> MALEVGDMEDGQLSDSDSDMTVAPSDRPLQLPKVLGGDSAMRAFQNTATACAPVSHYRAVESVDSSEESFSDSDDDSCLWKRKRQKCFNPPPKPEPFQFGQSSQKPPVAGGKKINNIWGAVLQEQNQDAVATELGILGMEGTIDRSRQSETYNYLLAKKLRKESQEHTKDLDKELDEYMHGGKKMGSKEEENGQGHLKRKRPVKDRLGNRPEMNYKGRYEITAEDSQEKVADEISFRLQEPKKDLIARVVRIIGNKKAIELLMETAEVEQNGGLFIMNGSRRRTPGGVFLNLLKNTPSISEEQIKDIFYIENQKEYENKKAARKRRTQVLGKKMKQAIKSLNFQEDDDTSRETFASDTNEALASLDESQEGHAEAKLEAE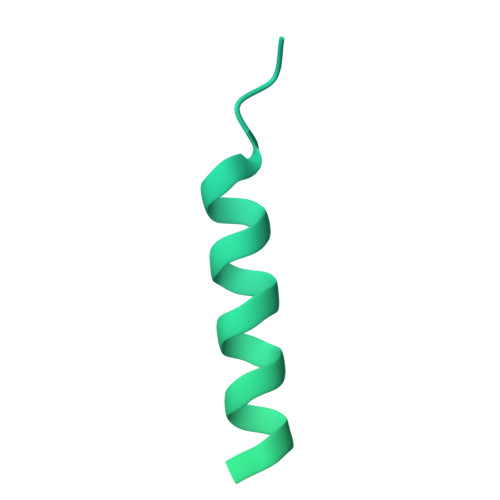EAIEVDHSHDLDIF Linafexor | 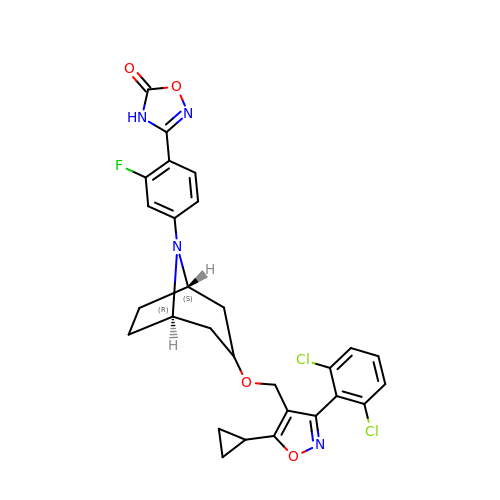C28 H25 Cl2 F N4 O4 | CEEANZUSISGCJL-VQFNDLOPSA-N> MTSEQTGEPAEDTSGVIKMAVKFDRRAYPAQITPKMCLLEWCRREKLAQPVYETVQRPLDRLFSSIVTVAEQKYQSTLWDKSAALAEQA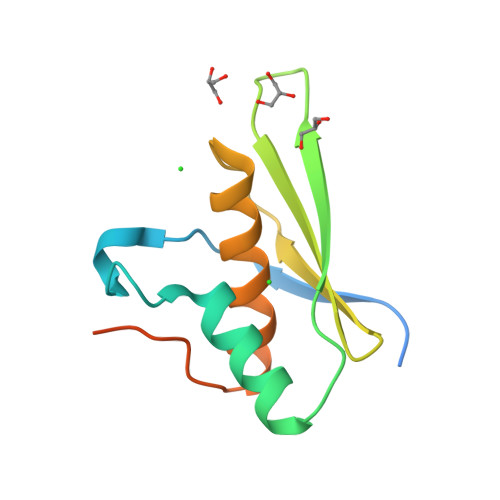AAIVCLRSQGLPEGRLGEESPSLHKHHHHHH UDP-di-N-acetyl-alpha-bacillosamine | 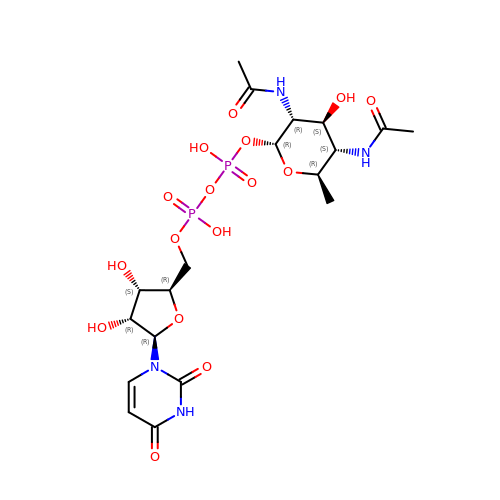C19 H30 N4 O16 P2 | KCAODEOZHCZEBC-TUHJILAWSA-N> MRFLPCIATLAATASALAIGDHVRSDDQYVLELAPGQTKVVTEAEKWALRAEGKRFFDITERASSLELASNKKQKLAVTYPDSVQHNETVQNLIKSLDKKNFETVLQPFSEFHNRYYKSDNGKKSSEWLQGKIQEIISASGAKGVTVEPF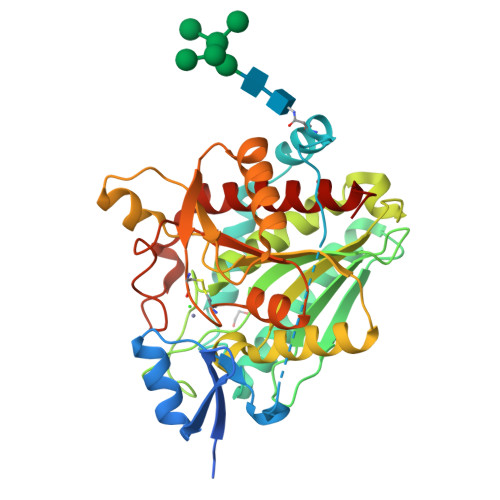KHSFPQSSLIAKIPGKSDKTIVLGAHQDSINLDSPSEGRAPGADDDGSGVVTILEAFRVLLTDEKVAAGEAPNTVEFHFYAGEEGGLLGSQDIFEQYSQKSRDVKAMLQQDMTGYTKGTTDAGKPESIGIITDNVDENLTKFLKVIVDAYCTIPTVDSKCGYGCSDHASATKYGYPAAFAFESAFGDDSPYIHSADDTIETVNFDHVLQHGRLTLGFAYELAFADSL>[2x]FSGYHIGVGRADCTGQVADINLMGYGKSGQNAQGILTRLYSRAFIMAEPDGSNRTVFVSIDIGMVSQRLRLEVLNRLQSKYGSLYRRDNVILSGTHTHSGPAGYFQYTVFVIASEGFSNQTFQHMVTGILKSIDIAHTNMKPGKIFINKGNVDGVQINRSPYSYLQNPQSERARYS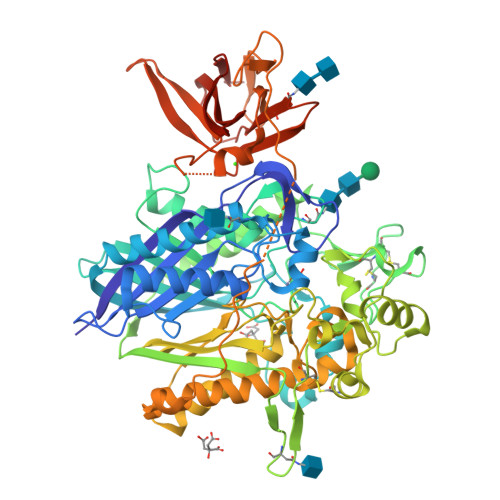SNTDKEMIVLKMVDLNGDDLGLISWFAIHPVSMNNSNHLVNSDNVGYASYLLEQEKNKGYLPGQGPFVAAFASSNLGDVSPNILGPRCINTGESCDNANSTCPIGGPSMCIAKGPGQDMFDSTQIIGRAMYQRAKELYASASQEVTGPLASAHQWVDMTDVTVWLNSTHASKTCKPALGYSFAAGTIDGVGGLNFTQGKTEGDPFWDTIRDQILGKPSEEIKECHKPKPILLHTGELSKPHPWHPDIVDVQIITLGSLAITAIPGEFTTMSGRRLREAVQAEFASHGMQNMTVVISGLCNVYTHYITTYEEYQAQRYEAASTIYGPHTLSAYIQLFRNLAKAIATDTVANLSRGPEPPFFKQLIVPLIPSIVDRAPKGRTFGDVLQPAKPEYRVGEVAEVIFVGANPKNSVQNQTHQTFLTVEKYEATSTSWQIVCNDASWETRFYWHKGLLGLSNATVEWHIPDTAQPGIYRIRYFGHNRKQDILKPAVILSFEGTSPAFEVVTIHHHHHH inosine diphosphate ribose | C15 H22 N4 O15 P2 | 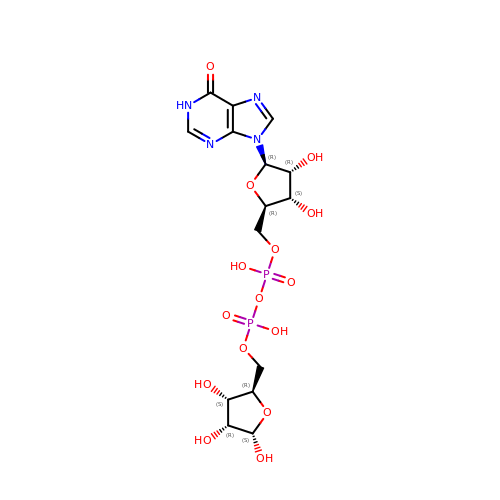GKBLKKRZILWFNP-ZQSHOCFMSA-N>GPHMHKVKLAAITCELPARSYENDDPVFAAVPDLSESWWQFWGVNRRGYFDPRNGENEFSLVVRAAERLLRSSDTAPDSVDMLICSASSPIMTDAGDVLPDLRGRLYPRMANVLSKQLGLSRALPLDSQMESASFLLNLRLAASMIRQGKAEKVLVVCSEYISNLLDFTSRTSTLFADGCAVALLTRGDDDSCDLLASAEHSDATFYEVATGRWRLPENPTGEAKPRLYFSLFSDGQNKMASFVPTNVPIAMRRALEKAGLGSDDIDYFVFHQPAPFLVKAWAEGIGARPEQYQLTMGDTGVMISVSIPYTLMTGLREGKIRPGDRIVMAGAATGWGFAAQVWQLGEVLVC[2x];>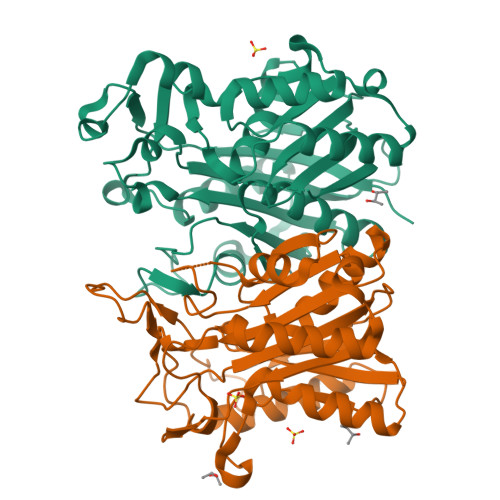[2x]MLIQAVGVNLPPSYVCLEGPLGGERPRAQGDEMLMQRLLPAVREALDEAAVKPEEIDLIVGLALSPDHLIENRDIMAPKIGHPLQKVLGANRAHVFDLTDSSLARALYVVDTLASDQGYRNVLVVRGESSQGLEVDSESGFALADGALALLCRPTGKAAFRRGALGGDPAQEWLPLSIPLNTDIRQVGDVKGHLNLPAQPGLPEAVRAGFTRLAGDFPQLNWVREEWFGQGRPDGRCLGPFELASQLRAAQRDRLDELLLISFDPFGMVVEGVTLELAGEAHA> MIKKAVLPVAGLGTRFLPASKSIPKEMVTVVDRPAIEYVVREAVEAGIEQIILVTHSSKASIENYFDRNFELETTLEQKKKFDLLAEITQIVP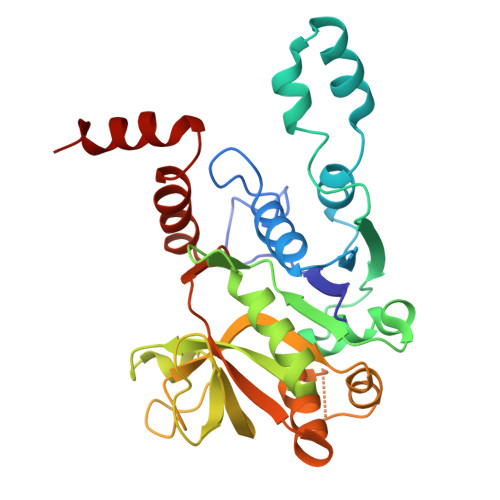EHVSVISVRQPQPLGLGHAVLCAKSVVGEDDFAVLLPDVLVKDGSGQNDLSRMISRYNSSQAAQIMVEAVPDHLVDQYGIVDVAQSPNEGESIAMQGIVEKPPVGAAPSNLSVVGRYVLPAKIMQLLENTPKGAGNEIQLTDAIAMLQDTDTVEAYRMQGQTFDCGSKLGYLKAVLHYGLEHPKLGMEFKQLILELK>SAYSTREILLALCIRDSRVHGNGTLHPVLELAARETPLRLSPEDTVVLRYHVLLEEIIERN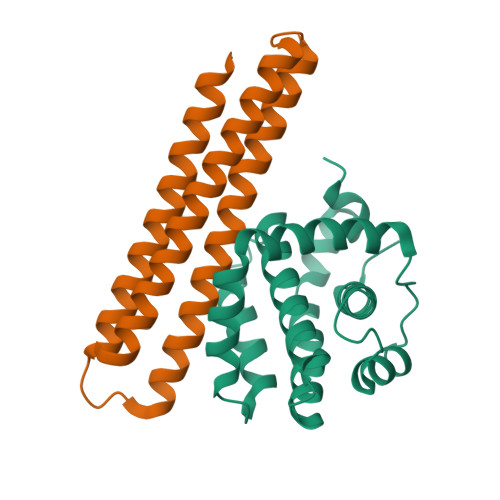SETFTETWNRFITHTEHVDLDFNSVFLEIFHRGDPSLGRALAWMAWCMHACRTLCCNQSTPYYVVDLSVRGMLEASEGLDGWIHQQGGWSTLIEDNI[2x];>ADPKKVLDKAKDQAENRVRELKQKLEELYKEARKLDLTQEMRRKLELRYIAAMLMAIGDIYNAIRQAKQEADKLKKAGLVNSQQLDELKRRLEELKEEASRKARDYGREFQLKLEYG[2x]> MSGLDKYLPGIEKLRRGDGEVEVKSLAGKLVFFY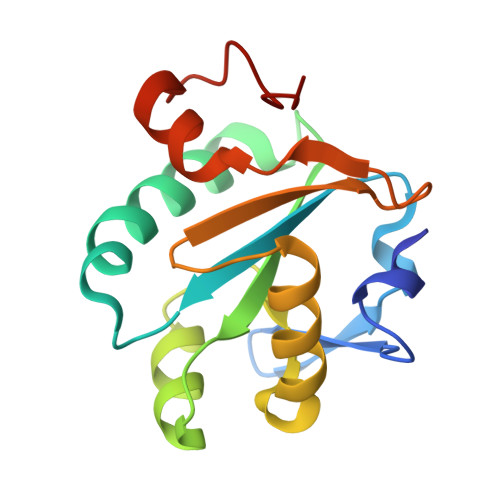FSASWCPPCRGFTPQLIEFYDKFHESKNFEVVFCTWDEEEDGFAGYFAKMPWLAVPFAQSEAVQKLSKHFNVESIPTLIGVDADSGDVVTTRARATLVKDPEGEQFPWKDAP>[2x]GSMKKERVITEFWDGKIIMVSPDDPKYALKKAEEVRELVDSELGFQQVSLRCPSQTRTYMFVSNEKKIVGCLIAEPIREAYR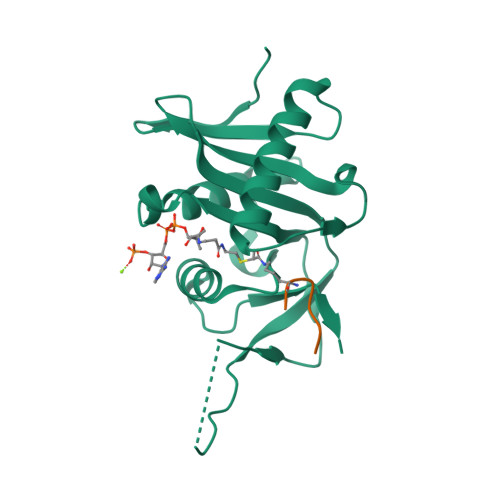VLAEPPSLHSLHGEPLERHRAWRCSTEPEPAICGISRIWVFALMRRKAIASRMVDAVRSSFMYGSVLTTEEIAFSDPTPDGKLFASTYCKVPDFLVYNFVS;>[2x]VIGAKKA> ASEIELVFRPHPTLMEKDDSAQTRYIKTSGNATVDHLSKYLAVRLALEELRSKGESNQMNLDTASEKQYTIYIATASGQFTVLDGSFSLELVSEKYWK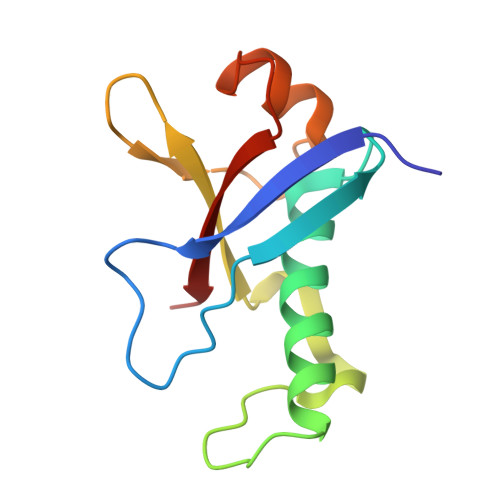VNKPMELYYAPTK3-fluoro-N-(3-hydroxy-4-methylphenyl)benzamide | C14 H12 F N O2 | 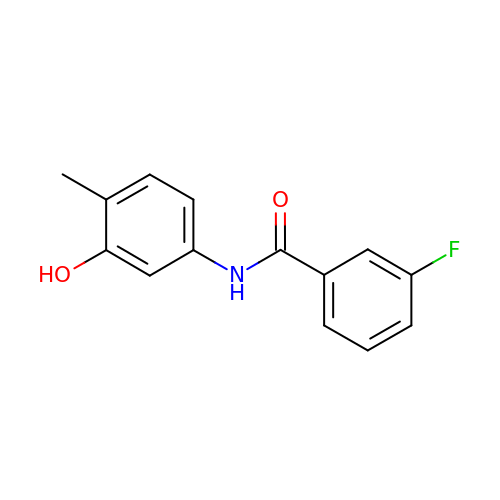HSWJYBWHEHPWSP-UHFFFAOYSA-N>ATTCATT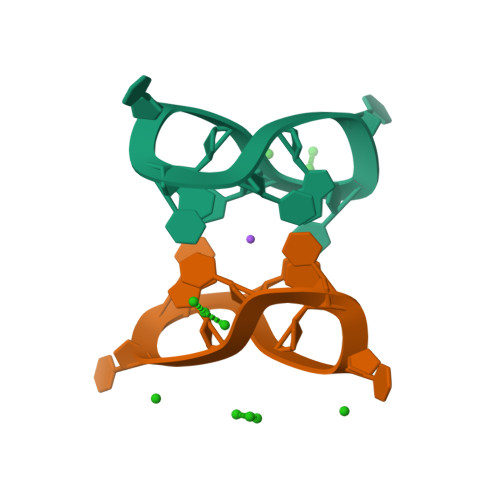C[2x]> MEHVAFG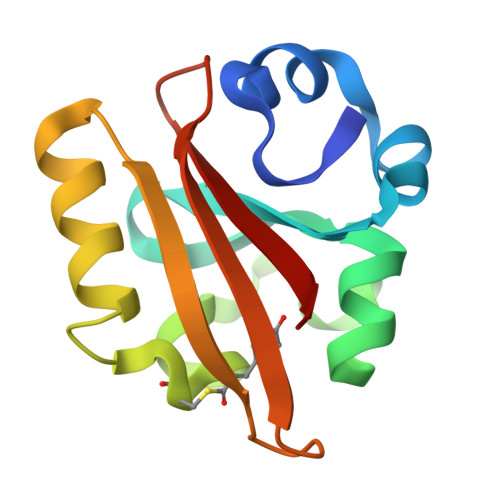SEDIENTLAKMDDGQLDGLAFGAIQLDGDGNILQYNAAESDITSRDPKQVIGKNFFKDVAPCTDSPEFYGKFKEGVASGNLNTMFEYTFDYQMTPTKVKVHMKKALSGDSYWVFVKRV>[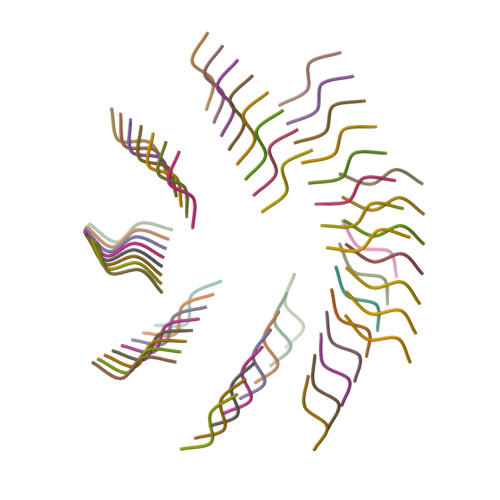62x]YAWF> GDPVEDIIHDALGSTARRAISSVTNAESAANTTPSSHRLETGRVPALQAAETGATSNATDENMIETRCVVNRNGVLETTINHFFSRSGLVGVVNLTDGGTDTTGYATWDIDIMGFVQLRRKCEMFTYMRFNAEFTFVTTTKNGEARPYMLQYMYVPPGAPKPTGRDAFQWQTATNPSVFVKLTDPPAQVSVPFMSPASAYQWFYDGYPTFGQHPETSNTTYGLCPNNMMGTFAVRVVSREASQLKLQTRVYMKLKHVRAWVPRPIRSQPYLLKNFPNYDSSKITNSARDRSSIKQANM;> SPSVEACGYSDRVAQLTVGNSSITTQEAANIVLAYGEWPEYCPDTDATAVDKPTRPDVSVNRFYTLDSKMWQENSTGWYWKFPDVLNKTGVFGQNAQFHYLYRSGFCLHVQCNASKFHQGALLVAVIPEFVIAGRGSNTKPNEAPHPGFTTTFPGTTGATFHDPYVLDSGVPLSQALIYPHQWINLRTNNCATVIVPYINAVPFDSAINHSNFGLIVIPVSPLKYSSGATTAIPITITIAPLNSEFGGLRQAVSQ;> GIPAELRPGTNQFLTTDDDTAAPILPGFTPTPTIHIPGEVHSLLELCRVETILEVNNTTEATGLTRLLIPVSSQNKADELCAAFMVDPGRIGPWQSTLVGQICRYYTQWSGSLKVTFMFTGSFMATGKMLVAYSPPGSAQPANRETAMLGT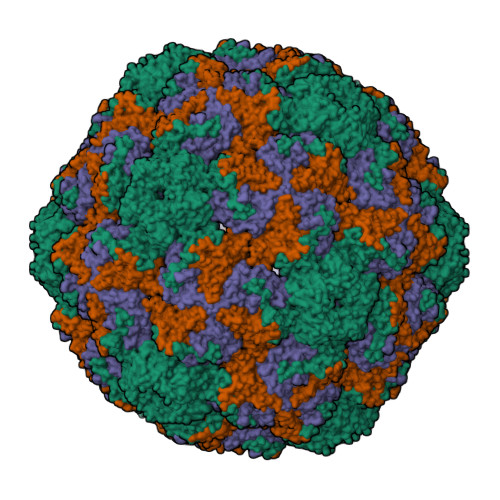HVIWDFGLQSSVSLVIPWISNTHFRTAKTGGNYDYYTAGVVTLWYQTNYVVPPETPGEAYIIAMGAAQDNFTLKICKDTDEVTQQAVLQ>[10x]MNVIAILNHMGVYFKEEPIRELHRALERLNFQIVYPNDRDDLLKLIENNARLCGVIFDWDKYNLELCEEISKMNENLPLYAFANTYSTLDVSLNDLRLQISFFEYALGAAEDIANKIKQTTDEYINTILPPLTKALFKYVREGKYTFCTPGHMGGTAFQKSPVGSLFYDFFGPNTMKSDISISVSELGSLLDHSGPHKEAEQYIARVFNADRSYMVTNGTSTANKIVGMYSAPAGSTILIDRNCHKSLTHLMMMSDVTPIYFRPTRNAYGILGGIPQSEFQHATIAKRVKETPNATWPVHAVITNSTYDGLLYNTDFIKKTLDVKSIHFDSAWVPYTNFSPIYEGKCGMSGGRVEGKVIYETQSTHKLLAAFSQASMIHVKGDVNEETFNEAYMMHTTTSPHYGIVASTETA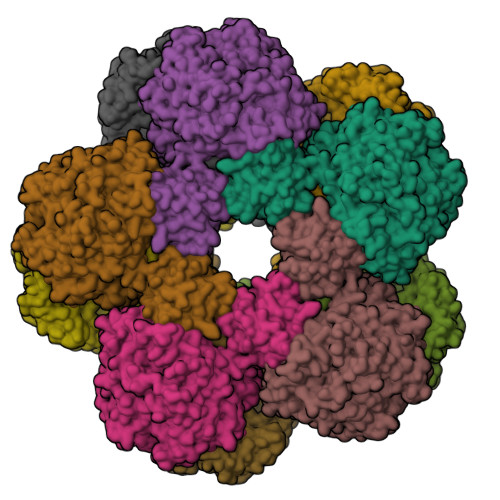AAMMKGNAGKRLINGSIERAIKFRKEIKRLRTESDGWFFDVWQPDHIDTTECWPLRSDSTWHGFKNIDNEHMYLDPIKVTLLTPGMEKDGTMSDFGIPASIVAKYLDEHGIVVEKTGPYNLLFLFSIGIDKTKALSLLRALTDFKRAFDLNLRVKNMLPSLYREDPEFYENMRIQELAQNIHKLIVHHNLPDLMYRAFEVLPTMVMTPYAAFQKELHGMTEEVYLDEMVGRINANMILPYPPGVPLVMPGEMITEESRPVLEFLQMLCEIGAHYPGFETDIHGAYRQADGRYTVKVLKE> NLSDIIEKETGKQLVIQESILMLPEE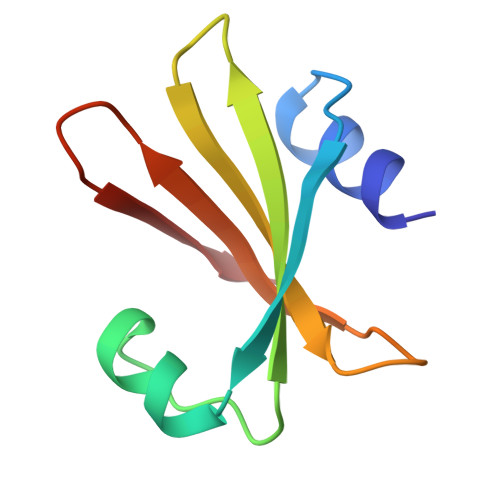VEEVIGNKPESDILVHTAYDESTDENVMLLTSDAPEYKPWALVIQDSNGENKIKML> RICFNQHSSQPQTTKTCSPGESSCYHKQWSDFRGTIIER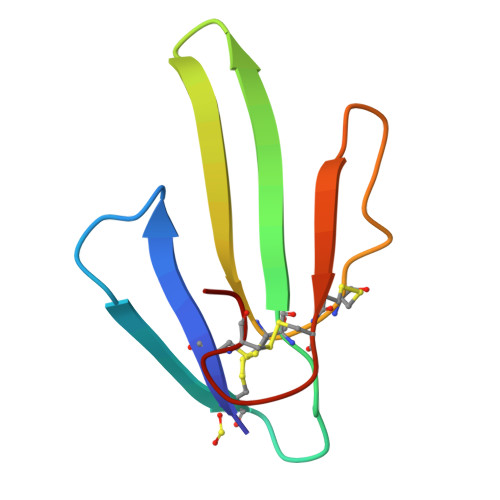GCGCPTVKPGIKLSCCESEVCNN4,5-dihydroxy-9,10-dioxo-9,10-dihydroanthracene-2-carboxylic 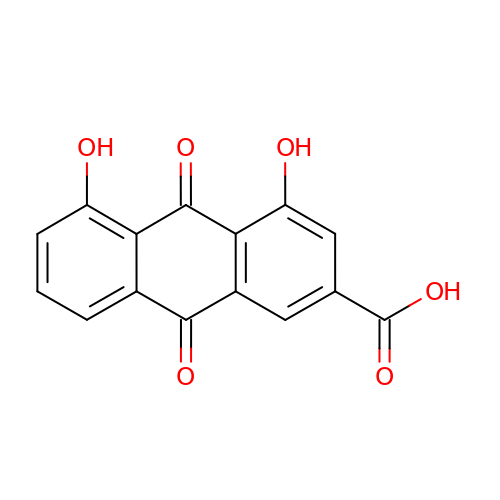acid | C15 H8 O6 | FCDLCPWAQCPTKC-UHFFFAOYSA-N ethyl 5-hydroxy-4-(morpholin-4-ylmethyl)-2-phenyl-1-benzofuran-3-carboxylate | C22 H23 N O5 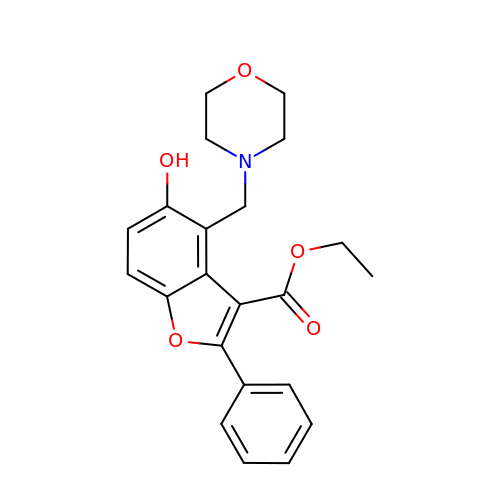| OGXGATRCXHSTEV-UHFFFAOYSA-N Our interest centers on 2-succinyl-5-enolpyruvyl-6-hydroxy-3-cyclohexadiene-1-carboxylate (SEPHCHC) synthase (EC 2.2.1.9) called MenD, the enzyme that catalyzes the first committed step of the classical menaquinone biosynthetic route. Subsequent studies revealed that MenD is a monofunctional SEPHCHC synthase and the only enzyme known to catalyze addition of a ThDP intermediate to the β-carbon of a second substrate, in a Stetter-like reaction, which is a 1,4-conjugate addition of an aldehyde to a β-unsaturated compound. MenD shows the three-domain architecture typical of ThDP-dependent enzymes.21 Sequence and structural analyses place MenD in the pyruvate oxidase class of these enzymes, where domain I contains the cofactor pyrimidine-binding motif, domain III binds the diphosphate, and the central domain has variable, often ill-defined, function. Oligomerization is essential for the function of ThDP-dependent enzymes, with each active site formed from two subunits.

We now report the medium-resolution crystal structure of the B. subtilis enzyme (BsMenD), solved by targeting the anomalous dispersion signal from a selenomethionine (SeMet) derivative. BsMenD crystallizes in an orthorhombic system, space group P212121, with four polypeptide chains, labeled A to D in the asymmetric unit. The structure was solved by use of single-wavelength anomalous diffraction (SAD) methods and refined to 2.35 Å resolution. Size-exclusion chromatography indicated that BsMenD consists of a mixture of dimer and tetramer in solution, with the dimer being much more abundant. Dimerization is essential for formation of the cofactor binding and active site, with residues from domain I of subunit A and domain III from subunit B forming one site (and vice versa, leading to two active sites per dimer). A metal cation, assigned as Mn2+, is bound and helps to position the diphosphate group of ThDP and so tether one part of the cofactor to the protein. In BsMenD, the side chains of Asp457 and Asn484, the main-chain carbonyl of Gly486, a water molecule, and two oxygen atoms from the diphosphate group form an octahedral coordination sphere about the metal ion. Almost all ThDP-dependent enzymes have a glutamate interacting with N1′ of the pyrimidine; Glu54 fulfills this role in BsMenD. The active site is polar, primarily basic due to the presence of four arginine residues (32A, 106A, 409B, and 428B) and a lysine (299B). A hydrophobic patch is formed by Ile489B, Phe490B, and Leu493B.

>MGSSHHHHHHSSGENLYFQGHMLEMTVNPITHYIGSFIDEFALSGITDAVVCPGSRSTPLAVLCAAHPDISVHVQIDERSAGFFALGLAKAKQRPVLLICTSGTAAANFYPAVVEAHYSRVPIIVLTADRPHELREVGAPQAINQHFLFGNFVKFFTDSALPEESPQMLRYIRTLASRAAGEAQKRPMGPVHVNVPLREPLMPDLSDEPFGRMRTGRHVSVKTGTQSVDRESLSDVAEMLAEAEKGMIVCGELHSDADKENIIALSKALQYPILADPLSNLRNGVHDKSTVIDAYDSFLKDDELKRKLRPDVVIRFGPMPVSKPVFLWLKDDPTIQQIVIDEDGGWRDPTQASAHMIHCNASVFAEEIMAGLTAATRSSEWLEKWQFVNGRFREHLQTISSEDVSFEGNLYRILQHLVPENSSLFVGNSMPIRDVDTFFEKQDRPFRIYSNRGANGIDGVVSSAMGVCEGTKAPVTLVIGDLSFYHDLNGLLAAKKLGIPLTVILVNNDGGGIFSFLPQASEKTHFEDLFGTPTGLDFKHAAALYGGTYSCPASWDEFKTAYAPQADKPGLHLIEIKTDRQSRVQLHRDMLNEAVREVKKQWEL[4x]>TLWRCCQRVVGWVPVLFITFVVVWSYYAYVVELCVFTIFGNEENGKTVVYLVAFHLFFVMFVWSYWMTIFTSPASPSKEFYLSNSEKERYEKEFSQERQQEILRRAARALPIYTTSASKTIRYCEKCQLIKPDRAHHCSACDSCILKMDHHCPWVNNCVGFSNYKFFLLFLLYSLLYCLFVAATVLEYFIKFWTNELTDTRAKFHVLFLFFVSAMFFISVLSLFSYHCWLVGKNRTTIESFRAPTFSYGPDGNGFSLGASKNWRQV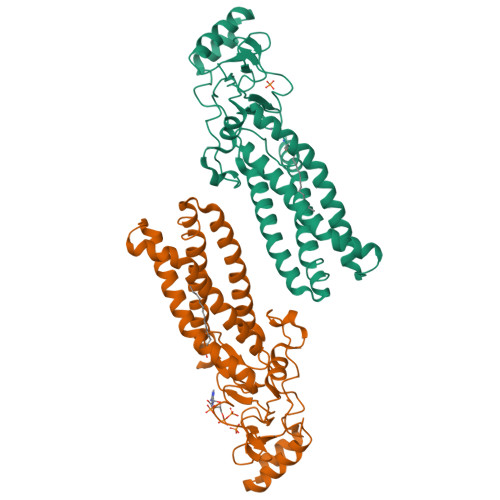FGDEKKYWLLPIFSSLGDGCSFPTRLVGM[2x]> AHMGCVSSKSTTVLSPQTSFNEASRTSFRALPGPSQRQLEVYDQCLIGAARWPDDSSKSNTPENRAYCQSMYNSIRSA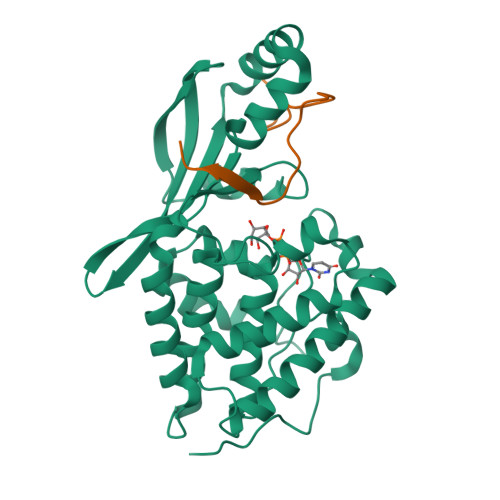GDEISRGGITSFEELWGRATEWRLSKLQRGEPLYSAFASERTSDTDAVTPLVKPYKSVLARVVDHEDAHDEIMQDNLFGDLNVKVYRQTAYLHGNVIPLNTFRVATDTEYLRDRVAHLRTELGAKALKQHLQRYNPDRIDHTNASYLPIIKDHLNDLYRQAISSDLSQAELISLIARTHWWAASAMPDQRGSAAKAEFAARAIASAHGIELPPFRNGNVSDIEAMLSGEEEFVEKYRSLLDSDCF;> APKFGDWDENNPSSADGYTHIFNKVRDEVD>TPDCVTGKVEYTKYNDDDTFTVKVGDKELF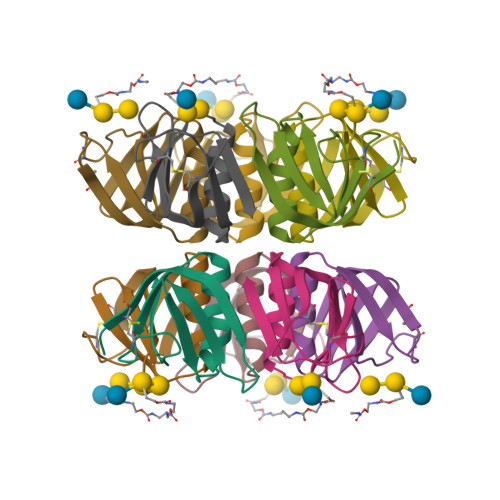TNRWNLQSLLLSAQITGMTVTIKTNACHNGGGFSEVIFR[5x]3-oxo-N-[(3S)-2-oxotetrahydrofuran-3-yl]decanamide | C14 H23 N O4 | 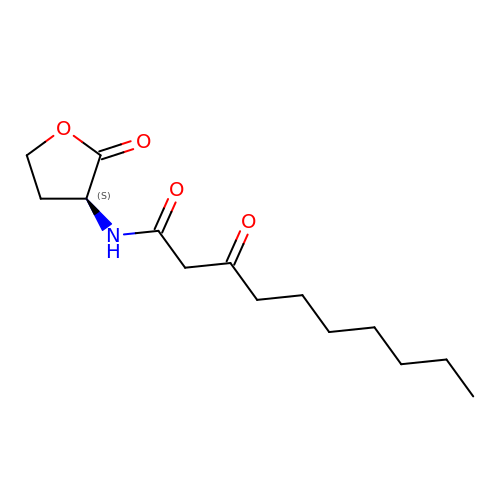KYGIKEQVUKTKRR-LBPRGKRZSA-N>MKGIIFN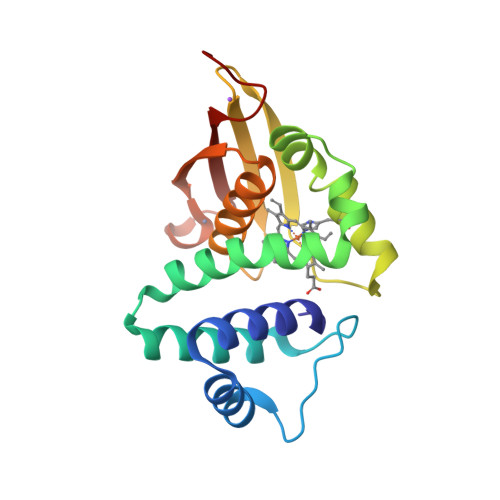VLEDMVVAQCGMSVWNELLEKHAPKDRVYVSAKSYAESELFSIVQDVAQRLNMPIQDVVKAFGQFLFNGLASRHTDVVDKFDDFTSLVMGIHDVIHLEVNKLYHEPSLPHINGQLLPNNQIALRYSSPRRLCFCAEGLLFGAAQHFAAAIQISHDTCMHTGADHCMLIIELQNDENLYFQ[2x]> MGFVRQIQLLLWKNWTLRKRQKIRFVVELVWPLSLFLVLIWLRNANPLYSHHECHFPNKAMPSAGMLPWLQGIFCNVNNPCFQSPTPGESPGIVSNYNNSILARVYRDFQELLMNAPESQHLGRIWTELHILSQFMDTLRTHPERIAGRGIRIRDILKDEETLTLFLIKNIGLSDSVVY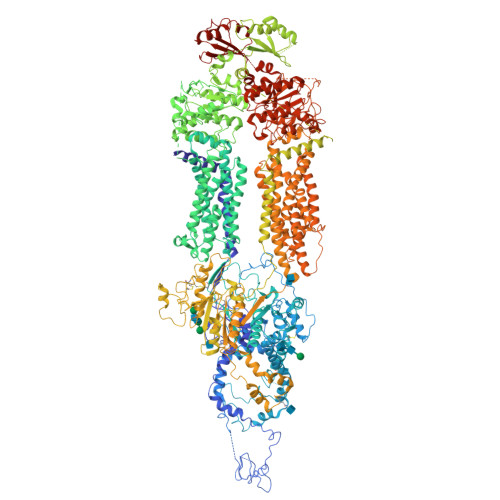LLINSQVRPEQFAHGVPDLALKDIACSEALLERFIIFSQRRGAKTVRYALCSLSQGTLQWIEDTLYANVDFFKLFRVLPTLLDSRSQGINLRSWGGILSDMSPRIQEFIHRPSMQDLLWVTRPLMQNGGPETFTKLMGILSDLLCGYPEGGGSRVLSFNWYEDNNYKAFLGIDSTRKDPIYSYDRRTTSFCNALIQSLESNPLTKIAWRAAKPLLMGKILYTPDSPAARRILKNANSTFEELEHVRKLVKAWEEVGPQIWYFFDNSTQMNMIRDTLGNPTVKDFLNRQLGEEGITAEAILNFLYKGPRESQADDMANFDWRDIFNITDRTLRLVNQYLECLVLDKFESYNDETQLTQRALSLLEENMFWAGVVFPDMYPWTSSLPPHVKYKIRMDIDVVEKTNKIKDRYWDSGPRADPVEDFRYIWGGFAYLQDMVEQGITRSQVQAEAPVGIYLQQMPYPCFVDDSFMIILNRCFPIFMVLAWIYSVSMTVKSIVLEKELRLKETLKNQGVSNAVIWCTWFLDSFSIMSMSIFLLTIFIMHGRILHYSDPFILFLFLLAFSTATIMLCFLLSTFFSKASLAAACSGVIYFTLYLPHILCFAWQDRMTAELKKAVSLLSPVAFGFGTEYLVRFEEQGLGLQWSNIGNSPTEGDEFSFLLSMQMMLLDAAVYGLLAWYLDQVFPGDYGTPLPWYFLLQESYWLGGEGCSTREERALEKTEPLTEETEDPEHPEGIHDSFFEREHPGWVPGVCVKNLVKIFEPCGRPAVDRLNITFYENQITAFLGHNGAGKTTTLSILTGLLPPTSGTVLVGGRDIETSLDAVRQSLGMCPQHNILFHHLTVAEHMLFYAQLKGKSQEEAQLEMEAMLEDTGLHHKRNEEAQDLSGGMQRKLSVAIAFVGDAKVVILDEPTSGVDPYSRRSIWDLLLKYRSGRTIIMSTHHMDEADLLGDRIAIIAQGRLYCSGTPLFLKNCFGTGLYLTLVRKMKNIQSQRKGSEGTCSCSSKGFSTTCPAHVDDLTPEQVLDGDVNELMDVVLHHVPEAKLVECIGQELIFLLPNKNFKHRAYASLFRELEETLADLGLSSFGISDTPLEEIFLKVTEDSDSGPLFAGGAQQKRENVNPRHPCLGPREKAGQTPQDSNVCSPGAPAAHPEGQPPPEPECPGPQLNTGTQLVLQHVQALLVKRFQHTIRSHKDFLAQIVLPATFVFLALMLSIVIPPFGEYPALTLHPWIYGQQYTFFSMDEPGSEQFTVLADVLLNKPGFGNRCLKEGWLPEYPCGNSTPWKTPSVSPNITQLFQKQKWTQVNPSPSCRCSTREKLTMLPECPEGAGGLPPPQRTQRSTEILQDLTDRNISDFLVKTYPALIRSSLKSKFWVNEQRYGGISIGGKLPVVPITGEALVGFLSDLGRIMNVSGGPITREASKEIPDFLKHLETEDNIKVWFNNKGWHALVSFLNVAHNAILRASLPKDRSPEEYGITVISQPLNLTKEQLSEITVLTTSVDAVVAICVIFSMSFVPASFVLYLIQERVNKSKHLQFISGVSPTTYWVTNFLWDIMNYSVSAGLVVGIFIGFQKKAYTSPENLPALVALLLLYGWAVIPMMYPASFLFDVPSTAYVALSCANLFIGINSSAITFILELFENNRTLLRFNAVLRKLLIVFPHFCLGRGLIDLALSQAVTDVYARFGEEHSANPFHWDLIGKNLFAMVVEGVVYFLLTLLVQRHFFLSQWIAEPTKEPIVDEDDDVAEERQRIITGGNKTDILRLHELTKIYPGTSSPAVDRLCVGVRPGECFGLLGVNGAGKTTTFKMLTGDTTVTSGDATVAGKSILTNISEVHQNMGYCPQFDAIDELLTGREHLYLYARLRGVPAEEIEKVANWSIKSLGLTVYADCLAGTYSGGNKRKLSTAIALIGCPPLVLLDEPTTGMDPQARRMLWNVIVSIIREGRAVVLTSHSMEECEALCTRLAIMVKGAFRCMGTIQHLKSKFGDGYIVTMKIKSPKDDLLPDLNPVEQFFQGNFPGSVQRERHYNMLQFQVSSSSLARIFQLLLSHKDSLLIEEYSVTQTTLDQVFVNFAKQQTESHDLPLHPRAAGASRQAQD>[10x]SAMDLPDVTLSLCGGLSENGEIS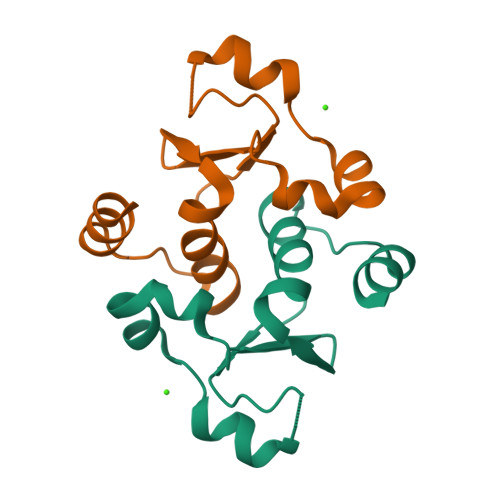KEKFMEHIITYHEFAENPGLIDNPNLVIRIYNRYYNWALAAPMILSLQVFQKSLPKATVESWVKDKMP> MLLGSSEESQAFQRQLTALIGYDVTDVSNVHDDELEFTRRGLVTPRMAEVASRDPKLYAMHPWVTSKPLPEYLWKKIANNCIFIVIHRSTTSQTIKVSPDDTPGAILQSFFTKMAKKKSLMDIPESQSEQDFVLRVCGRDEYLVGETPIKNFQWVRHCLKNGEEIHVVLDTPPDPALDEVRKEEWPLVDDCTGVTGYHEQLTIHGKDHESVFTVSLWDCDRKFRVKIRGIDIPVLPRNTDLTVFVEANIQHGQQVLCQRRTSPKPFTEEVLWNVWLEFSIKIKDLPKGALLNLQIYCGKAPALSSKASAESPSSESKGKVQLLYYVNLLLIDHRFLLRRGEYVLHMWQISGKGEDQGSFNADKLTSATNPDKENSMSISILLDNYCHPIALPKHQPTPDPEGDRVRAEMPNQLRKQLEAIIATDPLNPLTAEDKELLWHFRYESLKHPKAYPKLFSSVKWGQQEIVAKTYQLLARREVWDQSALDVGLTMQLLDCNFSDENVRAIAVQKLESLEDDDVLHYLLQLVQAVKFEPYHDSALARFLLKRGLRNKRIGHFLFWFLRSEIAQSRHYQQRFAVILEAYLRGCGTAMLHDFTQQVQVIEMLQKVTLDIKSLSAEKYDVSSQVISQLKQKLENLQ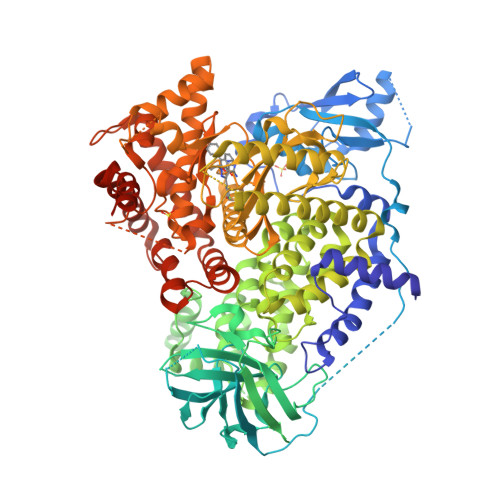NSQLPESFRVPYDPGLKAGALAIEKCKVMASKKKPLWLEFKCADPTALSNETIGIIFKHGDDLRQDMLILQILRIMESIWETESLDLCLLPYGCISTGDKIGMIEIVKDATTIAKIQQSTVGNTGAFKDEVLNHWLKEKSPTEEKFQAAVERFVYSCAGYCVATFVLGIGDRHNDNIMITETGNLFHIDFGHILGNYKSFLGINKERVPFVLTPDFLFVMGTSGKKTSPHFQKFQDICVKAYLALRHHTNLLIILFSMMLMTGMPQLTSKEDIEYIRDALTVGKNEEDAKKYFLDQIEVCRDKGWTVQFNWFLHLVLGIKQGEKHSAEFGLVPRGSGHHHHHH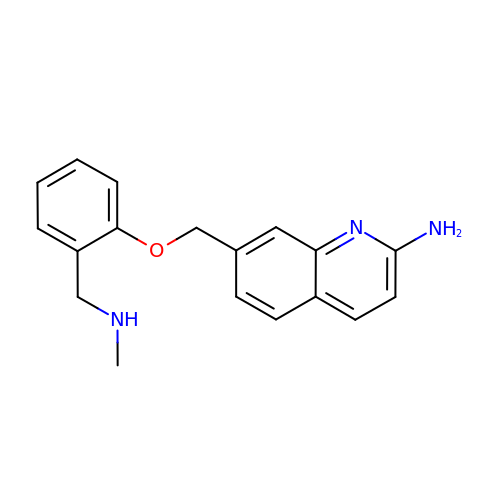7-[[2-(methylaminomethyl)phenoxy]methyl]quinolin-2-amine | C18 H19 N3 O | HZAOUJWVXIQVGZ-UHFFFAOYSA-N> GSHMRDHFALDRPSETHADYLLRTGQVVDISDTIYPRNPAM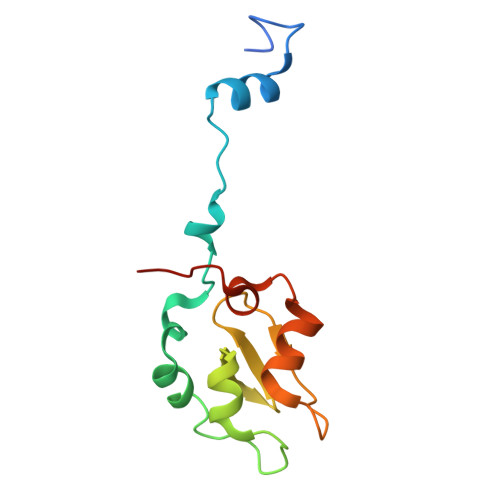YSEEARLKSFQNWPDYAHLTPRELASAGLYYTGIGDQVQCFACGGKLKNWEPGDRAWSEHRRHFPNCFFVLGRNLNIRSE>[2x]DGIYGSFENLKKHAGTMTLEAYMRFSA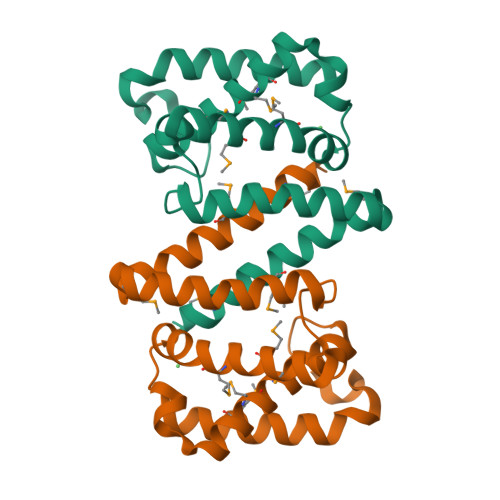KLSEAKDEMGTKEYEVFTKELKKLTNAKLAYGDSNGNIDYDALSSEKREEMKKVSMGLQPYFDKLNGHKSSKEVLTQEEFDRYMEALMTHEIVRVKTKSTGAIKVEEIPEAYKERFIKAEQFMEYVDEKVR>QGPLGSKLSEHLRYCDSILREMLSKKHAAYAWPFYKPVDAEALELHDYHDIIKHPMDLSTVKRKMDGREYPDAQGFAADVRLMFSNCYKYNPPDHEVVAMARKLQDVFEMRFAKMPDEP[2x];> XWKQWKKYGL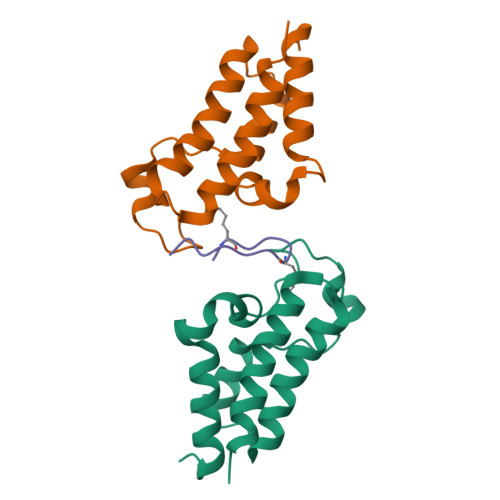KICX>[3x]MRTRSTISTPNGITWYYEQEGTGPDVVLVPDGLGECQMFDSSVSQIAAQGFRVTTFDMPGMSRSAKAPPETYTEVTAQKLASYVISVLDALDIKHATVWGCASGASTVVALLLGYPDRIRNAMCHELPTKLLDHLS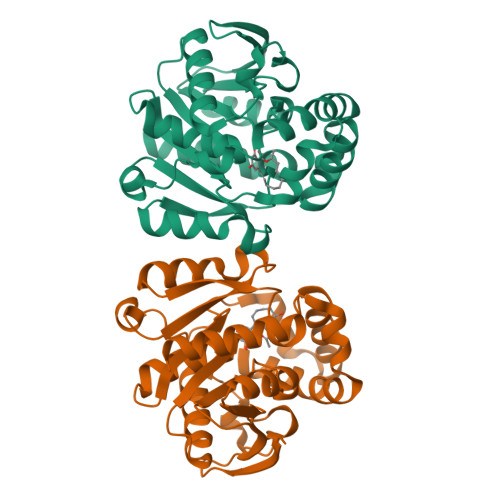NTAVLEDEEISKILANVMLNDVSGGSEAWQAMGDEVHARLHKNYPVWARGYPRTIPPSAPVKDLEALRGKPLDWTVGAATPTESFFDNIVTATKAGVNIGLLPGMHFPYVSHPDVFAKYVVETTQKHL> RRFLPSSVAAWGAGRVLQCAAEWYHMPGWKTQSSTKDARSREQRERDRKARQIEKLPRPEALHDFQYPYEKTILSDSMFEYPVYETELDTPQLFNLTPPPDFFIYWNATDFDRTAYPPVPEDDHRVLVPSSQSPRWIEH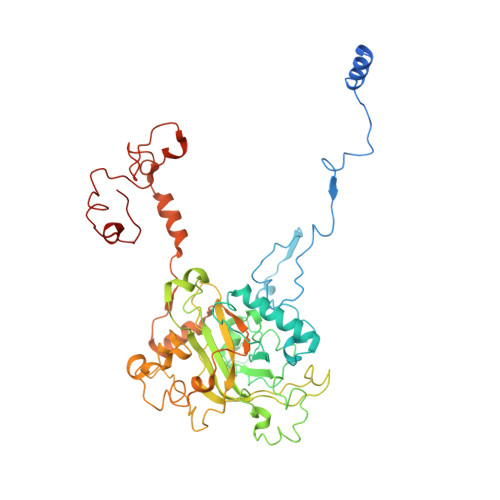RARLLQYLRKHEIMPHYVPHIHANVNLSVVFPGQYNTRARLTDENGDKIPPPPAQTKMTPRNFWFTAHCGNYMELTDVQQPPSVFFFEEAPAAASAASDAGEAGDAANKQSSHAAVNYYTFVMLSPDYPYRVPLLQDRHKADRGFFLNYMVANLRAPQAVSTVDGAVVDTEGLQSKGDVVVPYVAPLPTEDAGTTRHLCLLFKQTGHVPSVKPMTATEEQRDFPLAQRSNYRLHSALTKQTGLKMPPSASTACLASLRSVERAIPADPCAVSFFTTKWDIQVQEYYEKVGLPEPAAPVDEEIEALLEFHAMRPEKLRVRARHRPDGSVNMGDDPNFWAQALPTRAMDGSMQRGLGWSRRTTMGANGVPVVYPH> MSTIPSEIINWTILNEIISMDDDDSDFSKGLIIQFIDQAQTTFAQMQRQLDGEKNLTELDNLGHFLKGSSAALGLQRIAWVCERIQNLGRKMEHFFPNKTELVNTLSDKSIINGINIDEDDEEIKIQVDDKDENSIYLILIAKALNQSRLEFKLARIELSKYYNTNL;> TTSEKVFPKINVLIVEDNVINQAILGSFLRKHKISYKLAKNGQEAVNIWKEGGLHLIFMDLQLPVL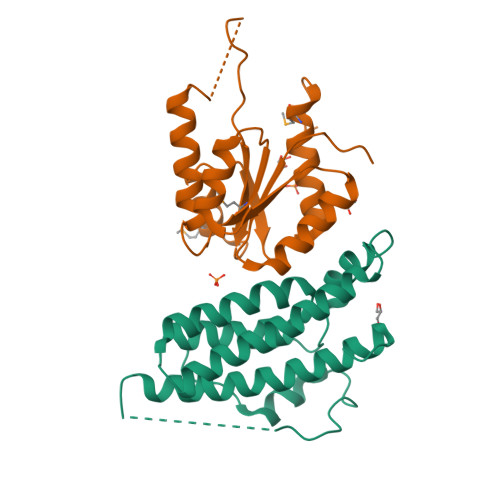SGIEAAKQIRDFEKQNGIGIQKSLNNSHSNLEKGTSKRFSQAPVIIVALTASNSQMDKRKALLSGCNDYLTKPVNLHALSKKITEWGCMQALIDFDSWKQGESRMTDSVLVKSPQKPIAPSNPHSFKQATSMTPTHSPVRKNSNLSPTQIEL>MSTKAIYPGTFDPITNGHIDIVTRAASMFDKVVLAIAASPSKKPMFSLDERIALAEQATAHLVNVEVIGFSDLMANFARAQQANILIRGLRAVADFEYEMQLAHMNRHLMPTLESVF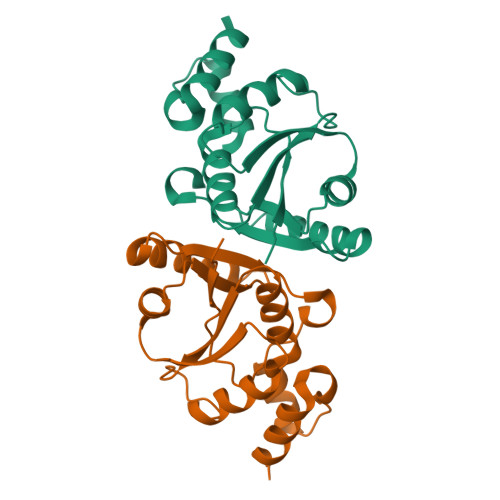LMPCKEWSFISSSLVKEVARHQGDVSHFLPANVHQALLNKLK[3x]> SNAMEKDIKRQIQILEIITSEEKWFTTIEISKILRCCNKTIMKDISFIKDFLPEDWHIKIKKGKGVRIYLPYNKHRNEITFLLFRESLTFRILQHLFERETKTIATLAERLYIQVPSILPALKRVENYLKKFGLKLRKKPLRLEGDEVRIMIMYLDLYLKSYNDTEWPFEKLKKEVIFQYLGTLEESLGISLHVVSKRHLSFFIAILLKRKQQGYKVQLNRKFLYFNTETPDYVKIGRIFEKLEREFGVSL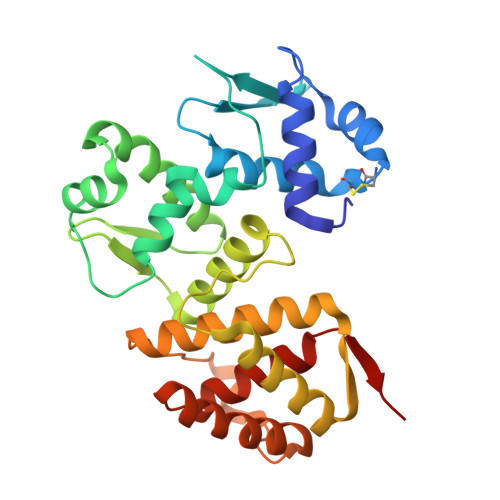TVQDKILLTISIKSSKYVYKDINK> PIFLNVLEAIEPGVVCAGHDNNQPDSFAALLSSLNELGERQLVHVVKWAKALPGFRNLHVDDQMAVIQYSWMGLMVFAMGWRSFTNVNSRMLYFAPDLVFNEYRMHKSRMYSQCVRMRHLSQEFGWLQITPQEFLCMKALLLFSIIPVDGLKNQKFFDELRMNYIKELDRIIACKRKNPTSCSRRFYQLTKLLDSVQPIARELHQFTFDLLIKSHMVSVDFPEMMAEIISVQVPKILSGKV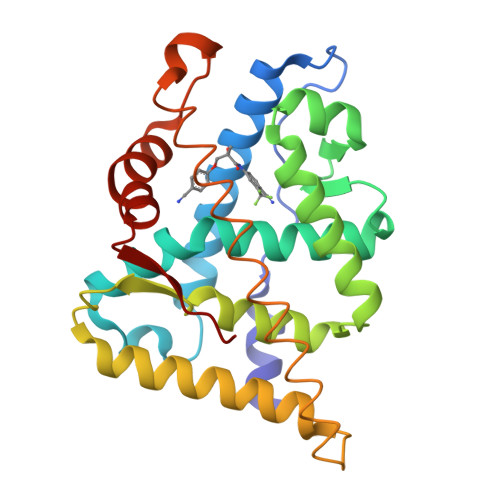KPIYFH>KTIIINGVQFNTDEDTTILKFARDNNIDISALCFLNNCNNDINKCEICTVEVEGTGLVTACDTLIEDGMIINTNSDAVNEKIKSRISQLLDIHEFKCGPCNRRENCEFLKLVIKYKARASKPFLPKDKTEYVDERSKSLTVDRTKCLLCGRCVNACGKNTETYAMKFLNKNGKTIIGAEDEKCFDDTNCLLCGQCIIACPVAALSEKSHMDRVKNALNAPEKHVIVAMAPSVRASIGELFNMGFGVDVTGKIYTALRQLGFDKIFDINFGADMTIMEAATELVQRIENNGPFPMFTSCCPGWVRQAENYYPELLNNLSSAKSPQQIFGTASKTYYPSISGLDPKNVFTVTVMPCTSKKFEADRPQMEKDGLRDIDAVITTRELAKMIKDAKIPFAKLEDSEADPAMGEYSGAGAIFGATGGVMEAALRSAKDFAENAELEDIEYKQVRGLNGIKEAEVEINNNKYNVAVINGASNLFKFMKSGMINEKQYHFIEVMACHGGCVNGG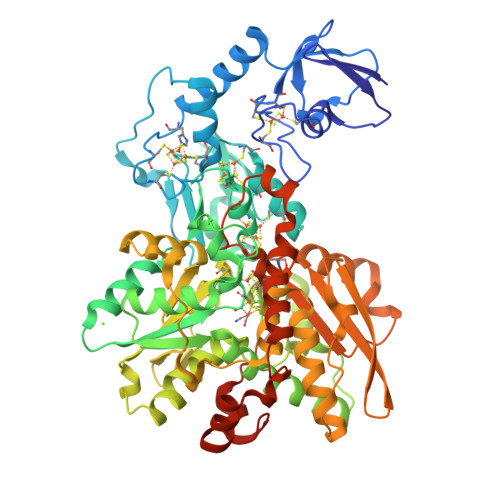GQPHVNPKDLEKVDIKKVRASVLYNQDEHLSKRKSHENTALVKMYQNYFGKPGEGRAHEILHFKYKKSAWSHPQFEK[2x]>AHFPQTPGFSGTLRPLRIEGDILDIEIEGEVPPQLNGTFHRVHPDAQFPPRFEDDQFFNGDGMVSLFRFHDGKIDFRQRYAQTDKWKVERKAGKSLFGAYRNPLTDDASVQGMIRGTANTNVMVHAGKLYAMKEDSPCLIMDPLTLETEGYTNFDGKLQSQTFCAHPKIDPVTGNLCAFAYGAKGLMTLDMAYIEISPTGKLLKEIPFQNPYYCMMHDFGVTEDYAVFAVMPLLSSWDRLEQRLPFFGFDTTLPCYLGILPRNGDARDLRWFKTGNCFVGHVMNAFNDGTKVHIDMPVSRNNSFPFFDVHGAPFDPVAGQGFLTRWTVDMASNGDSFEKTERLFDRPDEFPRIDERYATRAYRHGWMLILDTEKPYEAPGGAFYALTNTLGHIDLATGKSSSWWAGPRCAIQEPCFIPRSPDAPEGDGYVIALVDDHVANY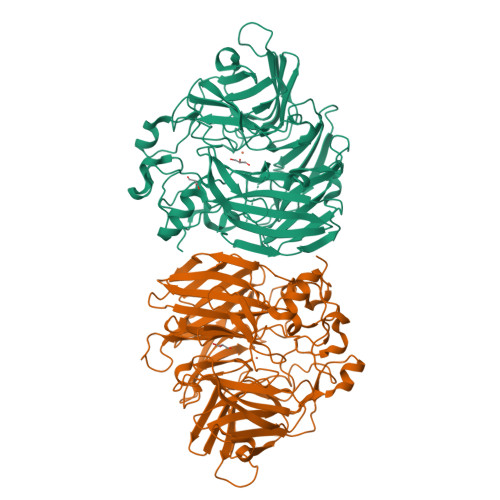SDLAIFDAQHVDQGPIARAKLPVRIRQGLHGNWADASRL[2x]>MSVEKIPGYTYGETENRAPFNLEDLKLLKEAVMFTAEDEEYIQKAGEVLEDQVEEILDTWYGFVGSHPHLLYYFTSPDGTPNEKYLAAVRKRFSRWILDTSNRSYDQAWLDYQYEIGLRHHRTKKNQTDNVESVPNIGYRYLVAFIYPFTATMKPFLARKGHTPEEVEKMYQAWFKATTL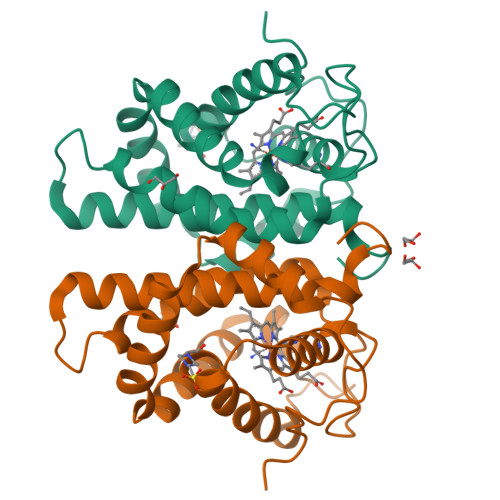QVALWSYPYVKYGDF[3x]> SCREKTELTPDQQTLLHFIMDSYNKQRMPQEITNKI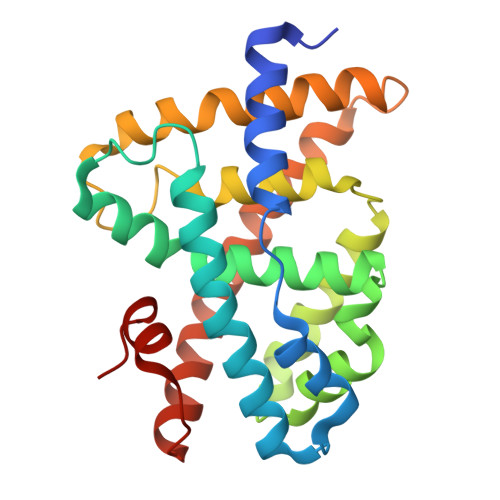LKEEFSAEENFLILTEMATNHVQVLVEFTKKLPGFQTLDHEDQIALLKGSAVEAMFLRSAEIFNKKLPSGHSDLLEERIRNSGISDEYITPMFSFYKSIGELKMTQEEYALLTAIVILSPDRQYIKDREAVEKLQEPLLDVLQKLCKIHQPENPQHFACLLGRLTELRTFNHHHAEMLMSWRVNDHKFTPLLCEIWDVQ2-(4-methoxyphenyl)-N-(pyridin-3-yl)acetamide 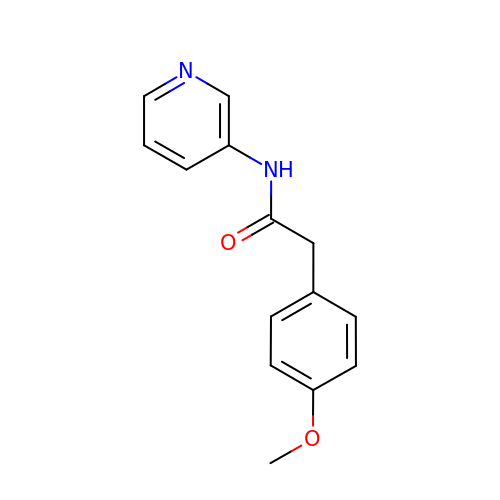| C14 H14 N2 O2 | MQUBBMQYRRRRDN-UHFFFAOYSA-N>[4x]MSAIQASWPSGTECIAKYNFHGTAEQDLPFCKGDVLTIVAVTKDPNWYKA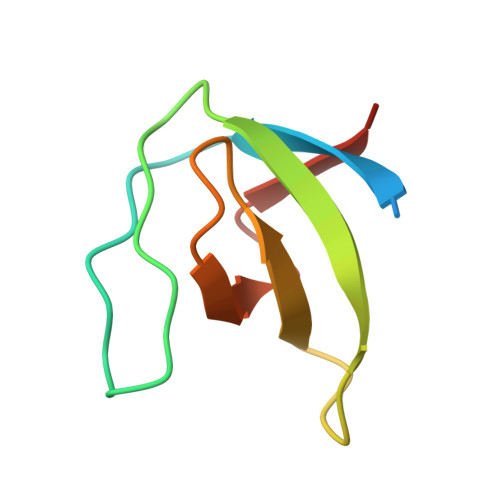KNKVGREGIIPANYVQKREGV> CACGTGGACAGGAG;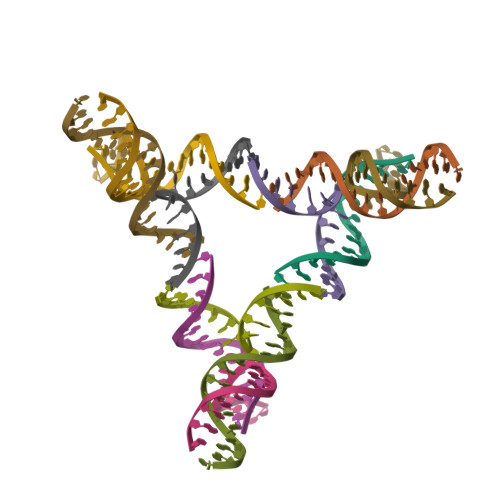> TGCTCCTGAGGTCGAGC;> CAGCTCAGCCTGACTCA;> GTGAGTCTCCACGT>[2x]DLYFQGGSGMQCEEKLEVFENGFKDEKFNVEVKFYGNDARKVLLAMIYELY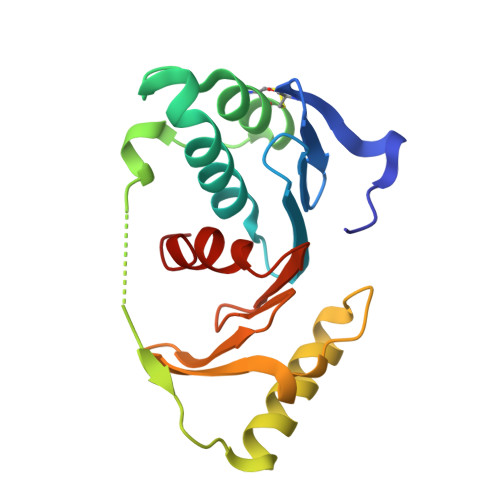LPEYGREYVYPFECAKEFWNIYLEGEEIQDEEFQLKPIKFTSEQVIKKLQEEIKKIKPPLEIKIEEAKIYKTKEGYLAVGNYFILDPRGRLFIFNKPSIANKILKYIWKW>SNAMTKSRFFSDVAETSSFVFAVAGADDEVVLETIRLALKQKLGKFLLFGKKEDKTLTANESVTWIQTDTAEAAAQGAILAVKNKEADILVKGFIPTATLMHHVLKKENGLRTDQLLSQIAIFDIPTYHKPLLITDCAMNVAPKTKEKIAITENALAVAHQIGITNPKIALLSAVEEVTAKMPSTLEAQEVVQHFGNQISVSGPLALDVAISKEAALHKGITDSSAGEADILIAPNIETGNALYKSLVYFAGAKVGSAVVGAK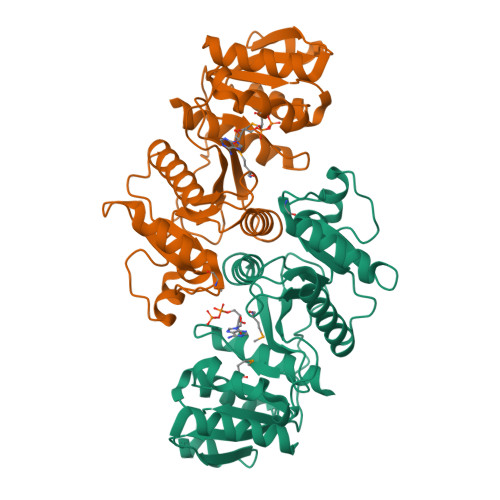VPIVISSRNDSPENKLASFILTVRLVEK[2x]2-Thiouridine (s2U) is a nucleobase modification that confers enhanced efficiency and fidelity both on modern tRNA codon translation and on nonenzymatic and ribozyme-catalyzed RNA copying. We have discovered an unusual base pair between two 2-thiouridines that stabilizes an RNA duplex to a degree that is comparable to that of a native A:U base pair. High-resolution crystal structures indicate similar base-pairing geometry and stacking interactions in duplexes containing s2U:s2U compared to those with U:U pairs. Notably, the C=O···H–N hydrogen bond in the U:U pair is replaced with a C=S···H–N hydrogen bond in the s2U:s2U base pair.

We also designed an RNA sequence, UU2, that forms a duplex with two adjacent U:U pairs, 5′-AGA GAA GUUC UUC UCU-3′, as well as its thiolated analog, SS2, 5′-AGA GAA Gs2Us2UC UUC UCU-3′. The UU1, UU2, and SS1 structures pack similarly, with one strand in each asymmetric unit forming a duplex with another strand in a different asymmetric unit. The U:U pairs in UU2 form two short hydrogen bonds between N3 of U8 and O4 of U9′, and between O2 of U8 and N3 of U9′ (2.8 and 2.8 Å). Considering the shorter hydrogen bonds in UU2, the modified s2U:s2U base pairs in SS2 presumably form weaker hydrogen bonds. At the same time, the sulfur atoms in SS2 have more surface exposed area compared with the corresponding oxygen atoms in UU2, which are buried in the minor groove. Interestingly, although both UU2 and SS2 duplexes maintain the A-form geometry with all nucleotides in the C3′-endo conformation, their structural parameters are slightly different. For instance, the opening of the s2U:s2U pairs (−4.81°/–1.48°) is much smaller than that of the native U:U pairs (12.83°). On the other hand, the twist on the U8–U9/U8′–U9′ step on UU2 is smaller than that on SS2 (20.63 vs 37.00°) to allow for the formation of the similarly packed adjacent UU pair. As a result, the overlap area of G7-U8/U9′-C10′ is much smaller in SS2 than that in UU2 (3.86 vs 11.04 Å2), indicating a weaker base stacking interaction. These observations suggest that at least in our crystal structures both the hydrogen bonding and base stacking interactions in SS2 are weaker than those in UU2.

> AGAGAAGUUCUUCUCU>[2x]MGQGPELHLASQFVNEACRALVFGGCVEKSSVSRNPEVPFESSAYRISASARGKELRLILSPLPGAQPQQEPLALVFRFGMSGSFQLVPREELPRHAHLRFYTAPPGPRLALCFVDIRRFGRWDLGGKWQPGRGPCVLQEYQQFRE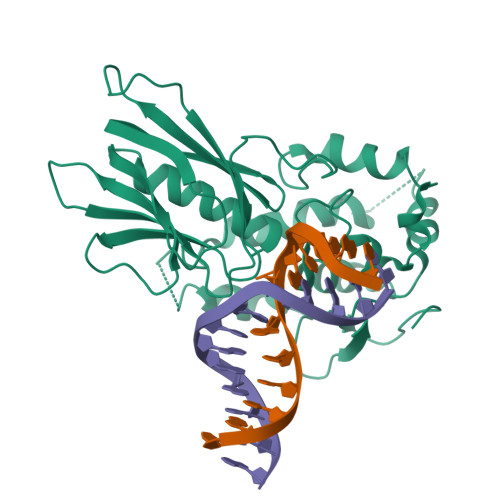NVLRNLADKAFDRPICEALLDQRFFNGIGNYLRAEILYRLKIPPFEKARSVLEALQQHRPSPELTLSQKIRTKLQNPDLLELCHSVPKEVVQLGGKGYGSESGEEDFAAFRAWLRCYGMPGMSSLQDRHGRTIWFQGDPGPLAPKGRKS> MNTRTIYLAGGCFWGLEAYFQRIDGVVDAVSGYANGNTKNPSYEDVSYRHTGHAETVKVTYDADKLSLDDILQYFFRVV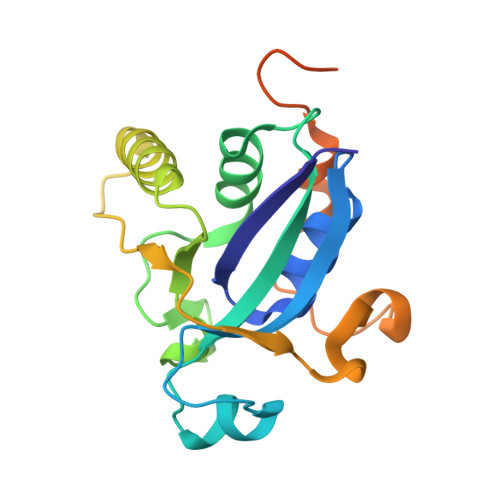DPTSLNKQGNDTGTQYRSGVYYTDPAEKAVIAAALKREQQKYQLPLVVENEPLKNFYDAEEYHQDYLIKNPNGYCHIDIRKADEPLPGKTKTAPQGKGFDAATYKKPSDAELKRT> GAMGSMTDDKDVLRDVWFGRIPTCFTLYQDEITEREAEPYYLLLPRVSYLTLVTDKVKKHFQKVMRQEDISEIWFEYEGTPLKWHYPIGLLFDLL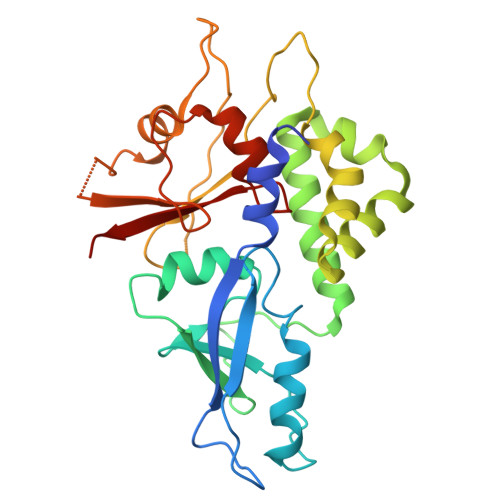ASSSALPWNITVHFKSFPEKDLLHCPSKDAIDAHFMSCMKEADALKHKSQVINEMQKKDHKQLWMGLQNDRFDQFWAINRKLMEYPAEENGFRYIPFRIYQTTTERPFIQKLFRPVAADGQLHTLGDLLKEVCPSAIDPEDGEKKNQVMIHGIEPMLETPLQWLSEHLSYPDNFLHISIIPQPTD>ATCYCRTGRCATRESLS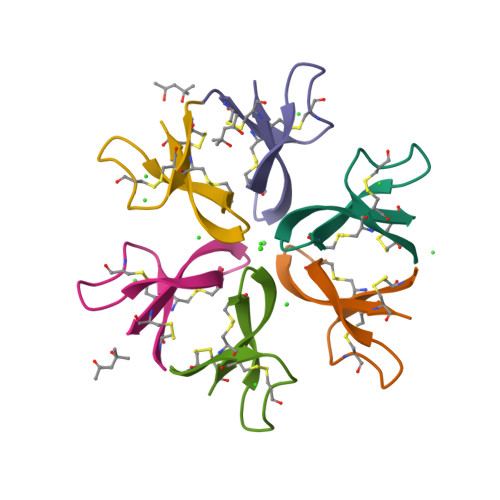GVCEISGRLARLCCR[6x]> MLTVIAEIRTRPGQHHRQAVLDQ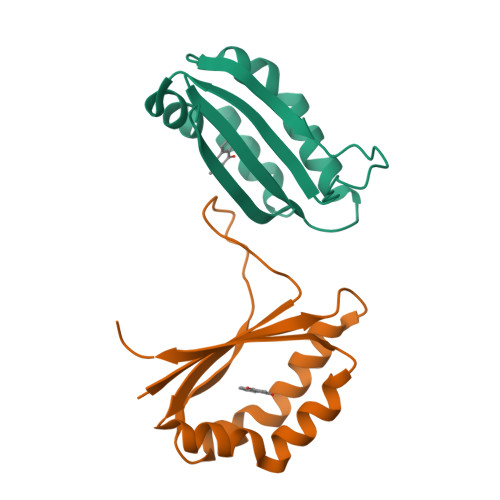FAKIVPTVLKEEGCHGYAPMVDCAAGVSFQSMAPDSIVMIEQWESIAHLEAHLQTPHMKAYSEAVKGDVLEMNIRILQPGISGRVHHHHHH4-amino-8-(4-aminophenyl)pyrido[2,3-d]pyrimidin-5(8H)-one | C13 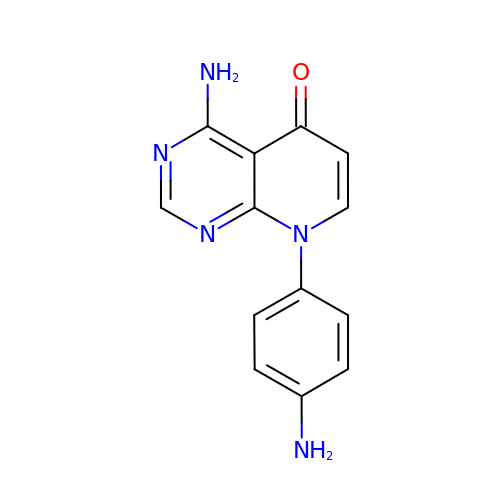H11 N5 O | VKOOVQQNRDYNBW-UHFFFAOYSA-N2-~{tert}-butyl-4-(furan-2-ylmethylamino)-~{N}-(2-methylpropyl)-~{N}-[(3~{S})-piperidin-3-yl]pyrimidine-5-carboxamide 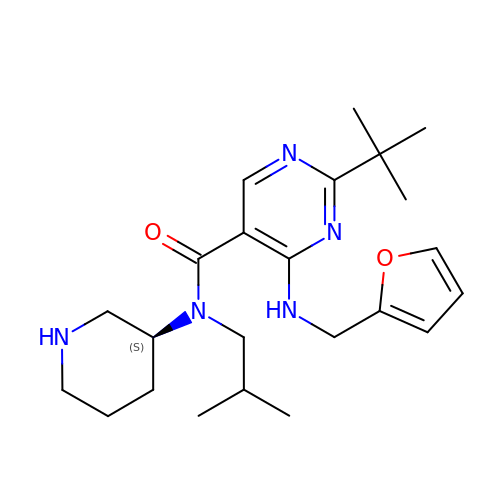| C23 H35 N5 O2 | RRLGPXVRIYOXIU-KRWDZBQOSA-N> MPVTINNF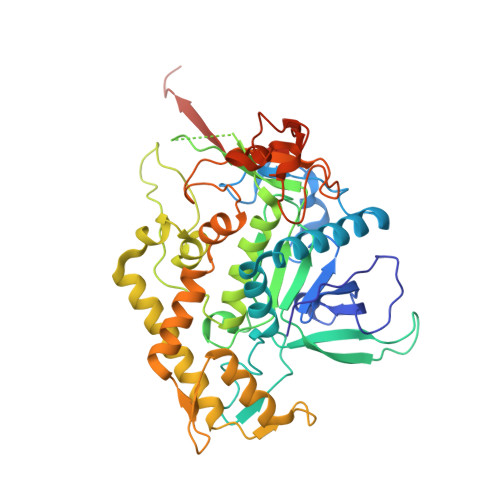NYNDPIDNNNIIMMEPPFARGTGRYYKAFKITDRIWIIPERYTFGYKPEDFNKSSGIFNRDVCEYYDPDYLNTNDKKNIFLQTMIKLFNRIKSKPLGEKLLEMIINGIPYLGDRRVPLEEFNTNIASVTVNKLISNPGEVERKKGIFANLIIFGPGPVLNENETIDIGIQNHFASREGFGGIMQMKFCPEYVSVFNNVQENKGASIFNRRGYFSDPALILMHELIHVLHGLYGIKVDDLPIVPNEKKFFMQSTDAIQAEELYTFGGQDPSIITPSTDKSIYDKVLQNFRGIVDRLNKVLVCISDPNININIYKNKFKDKYKFVEDSEGKYSIDVESFDKLYKSLMFGFTETNIAENYKIKTRASYFSDSLPPVKIKNLLDNEIYTIEEGFNISDKDMEKEYRGQNKAINKQAYEEISKEHLAVYKIQMCVDGIITSKTKSLIEGR> GGGCACUUACCCUUUAGUGCGAAGGUUUCGACCUUCGAUCCAUUUGUUCGCAAAUGGGAUGAUCUUCGGAUCAUCCGCGUAGUCUGUUCAGUCGUUUCGACGACUGGCCCCACUUCGGUGGGGCCACGGUACUUAGAAGUGAACACUAAGUGUCGUGAACACCAUUUGGUUAACUGCUCAAACUAAAUGGUGAUGAGGGAAGGAAUGACCCUCAUCGGACUACGCGAUCCGAGUGAUGGGAAUGGCUGACCCAUCGCUCGGCACUGGAGGGUGAGUGCCCCUCAUUCGCAUAAGGGCCGACCCAGACAACAGCCAAGUUUGGGUCGGAGAUGCGAACAUUCCACGCAUCUGAACGGUUGAGAACUUACAAGGGCAAGAGCAGAGUCCUUGUAAGGGCUUUACACGUCAAGUUCACAGACGUGUAAGGCCCGUCGCCCUUCGGGGCGACGUUCACGGCAUUUCGAUGCCGUGCAGC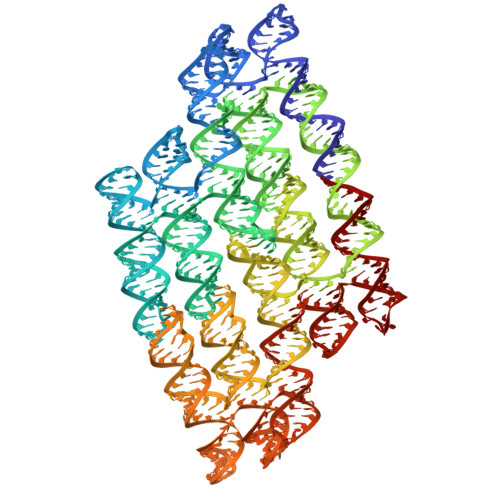CUGUUCGCAGGCUGCUUGACCGUUCCCCUGCCCUUUCGAGGGCAGACUACUCUUCGGAGUAGUCUUAUGUGAAUGAG2',3'-DIDEOXYCYTIDINE 5'-TRIPHOSPHATE | C9 H16 N3 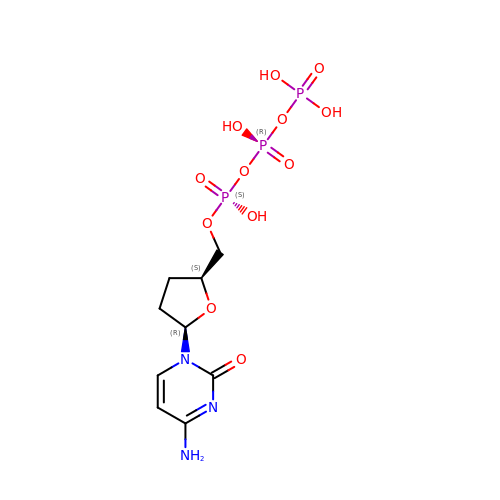O12 P3 | ARLKCWCREKRROD-POYBYMJQSA-N>IVGGYNCEENSVPYQVSLNSGYHFCGGSLINEQWVVSAGHCYKSRIQVRLGEHNIEVLEGNEQFIN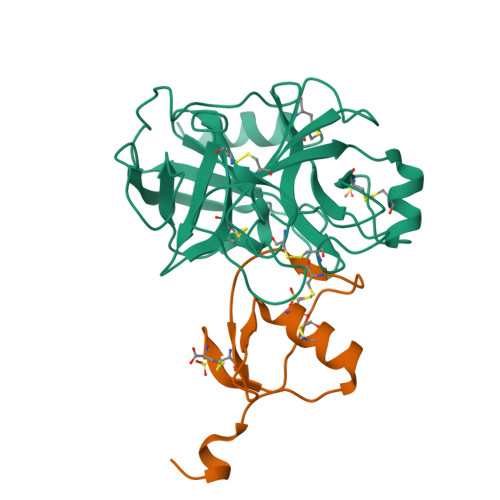AAKIIRHPQYDRKTLNNDIMLIKLSSRAVINARVSTISLPTAPPATGTKCLISGWGNTASSGADYPDELQCLDAPVLSQAKCEASYPGKITSNMFCVGFLEGGKDSCQGDAGGPVVCNGQLQGVVSWGDGCAQKNKPGVYTKVYNYVKWIKNTIAANS[2x];>[2x]GPGYLDSLGREAKCYSELNGCTKIYDPVCGTDGNTYPNECVLCFENRKRQTSILIQKSGPC>MAKTKGTASGRGGLGGQGAGGDVIEVGGAGQGGYGGLGSQGTSGRGGLGGQGAGGDVIEVGGAGQGGYGGLGSQGTSGRGGLGGQGAGGDVIEVGGAGQGGYGGLGSQGTSGRGGLGGQGAGGDVIEVGGAGQGGYGGLGSQGTSGRGGLGGQGAGGDVIEVGGAGQGGYGGLGSQGTSGRGGLGGQGAGGDVIEVGGAGQGGYGGLGSQGTSGRGGLGGQGAGGDVIEVGGAGQGGYGGLGSQGTSGRGGLGGQGAGGDVIEVGGAGQGGYGGLGSQGTSGRGGLGGQGAGGDVIEVGGAGQGGYGGLGSQGTSGRGGLGGQGAGGDVIEVGGAGQGGYGGLGSQGTSGRGGLGGQGAGGDVIEVG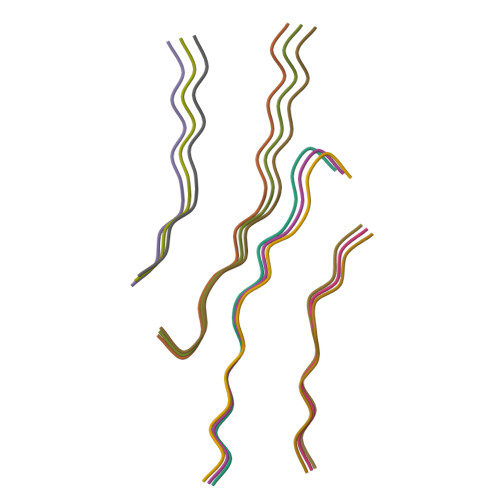GAGQGGYGGLGSQGTSGRGGLGGQGAGGDVIEVGGAGQGGYGGLGSQGTSGRGGLGGQGAGGDVIEVGGAGQGGYGGLGSQGTSGRGGLGGQGAGGDVIEVGGAGQGGYGGLGSQGTSGRGGLGGQGAGGDVIEVGGAGQGGYGGLGSQGTSGRGGLGGQGAGGDVIEVGGAGQGGYGGLGSQGTSSGHHHHHHHHHH[12x]> MAQEITWRNIGATVSPGSASSMSAGTTGVQQALGALGDIISRQQEMNVNNAKLQREANTQSYLDQVAASTLEQLSNADYRSGLEAQRDAMGMNLDRAATRDAI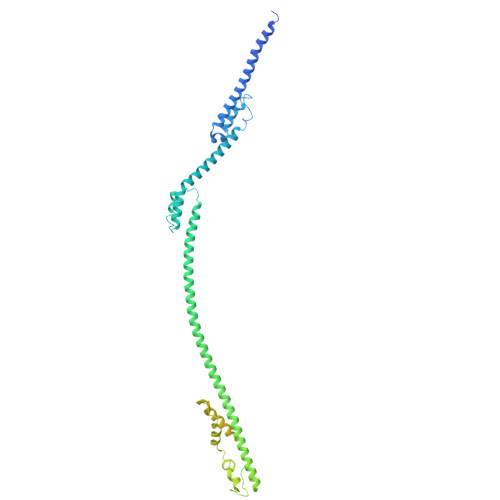TKQISAQQNQAAATQKFDDMQAEVGQRGIVDQLRTLSAEGRAGEVNQILAEQQLINEGEIRKELTGVQDAIQNRQYRAAGEQRAQAAANRAAEAHSLSMAAGRENLAFTREQRDELRRDRDEAKLVSGTIATTFQDYDESRQAQSEIMRIVGKEVGMPTDDQGMPDMSRASQDQLDAFSNALNEAGVQANTSPTERRNAVLKSLVDAGVSSKGIAQAKQEMELRESLEGLAPQDRTKVEATIGAVNAELDTLQRTATEDYEREVARNPFVEPDKDPLGSVNKIVDKAVKSGFGWEGDRQDLNNMLVDFATNGIKLPDGRTAVVPSKLLEQAFNTTNTWLFKNAGDVEKRIIELMTTDGMTQMREDAPTIRENFLKTVSDIANQKRSNAVKVTRSAEREKGVTMDPTDDLTFALRGRKR> SENYALTTNQGVR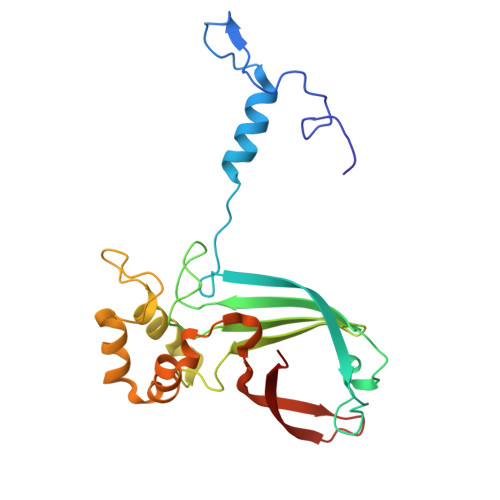IADDQNSLRAGSRGPTLLEDFILREKITHFDHERIPERIVHARGSAAHGYFQPYKSLSDITKADFLSDPNKITPVFVRFSTVQGGAGSADTVRDIRGFATKFYTEEGIFDLVGNNTPIFFIQDAHKFPDFVHAVKPEPHWAIPQGQSAHDTFWDYVSLQPETLHNVMWAMSDRGIPRSYRTMEGFGIHTFRLINAEGKATFVRFHWKPLAGKA>MGRGSHHHHHHGMAMNIKELSLHELCEELKTPAWNVPLTFVGDVGGTSARMGFVREGKNDSVHACVTRYSMKRKDITELIEFFNEIIELMPASVIK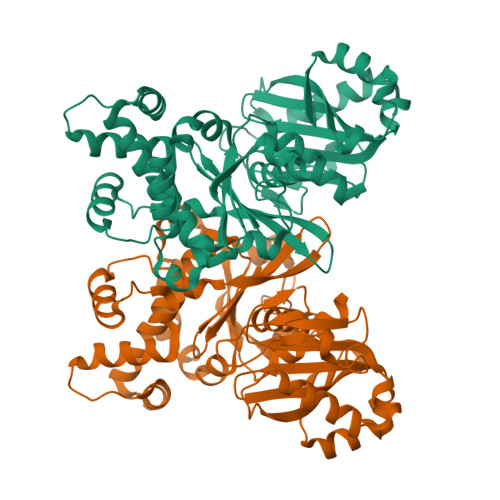RVKAGVINVPGPVTGGAVGGPFNNLKGIARLSDYPKALFPPGRSAILNDLEAGGFGVLAVSDAHVFSEYFGVMWEGTQWRTCEQEPAGSVIGRGRCLVLAPGTGLGSSLIYYNPMNQQHIVVPLELGSQTIPMRKDIDYIQTLHAELKLLPNYENMVSGAGLEFHYRQVVRGSRPPCSAGEIAKLASEGDANACKAMKKYHEYLMRVGSEASMALLPLTIVLVGDNIVNNAFFYRNPQNLKEMHREALNHEMERLGFQSRVTYLRQKKLLNLNLMGCYRCGLDLS[2x]> MQDCGLPPDVPNAQPALEGRTSFPEDTVITYKCEESFVKIPGEKDSVICLKGSQWSDIEEFCNRSCEVPTRLNSASLKQPYITQNYFPVGTVVEYECRPGYR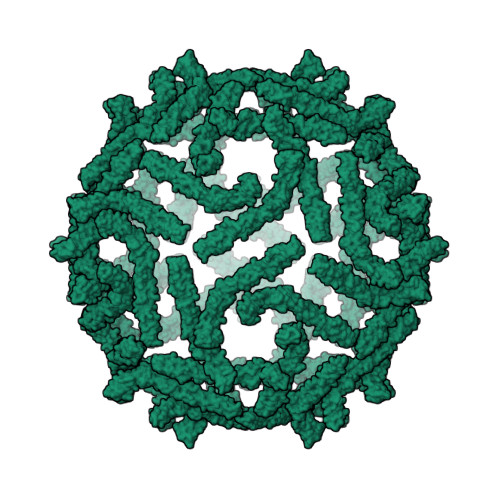REPSLSPKLTCLQNLKWSTAVEFCKKKSCPNPGEIRNGQIDVPGGILFGATISFSCNTGYKLFGSTSSFCLISGSSVQWSDPLPECREIYCPAPPQIDNGIIQGERDHYGYRQSVTYACNKGFTMIGEHSIYCTVNNDEGEWSGPPPECRGC> GAHMKSTFKSEYPFEKRKAESERIADRFKNRIPVICEKAEKSDIPEIDKRKYLVPADLTVGQFVYVIRKRIMLPPEKAIFIFVNDTLPPTAALMS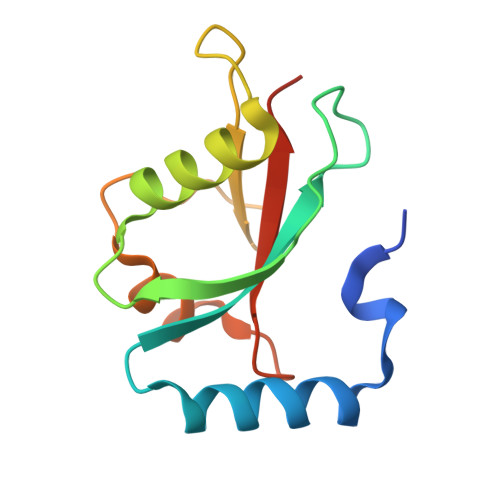AIYQEHKDKDGFLYVTYSGENTFG{2-[(1-benzofuran-2-ylsulfonyl)carbamoyl]-5-methoxy-1H-indol-1-yl}acetic 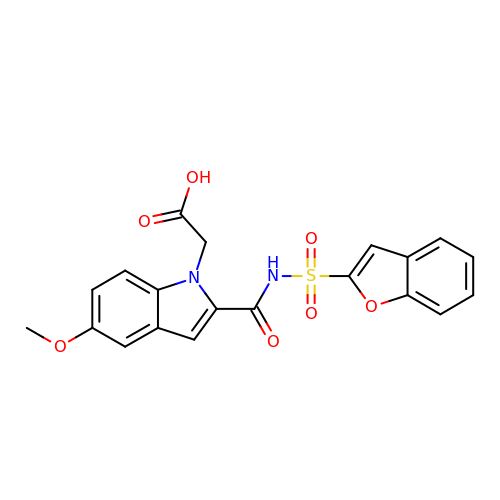acid | C20 H16 N2 O7 S | XOSVMFKSAWOSMH-UHFFFAOYSA-N>GPLGSGRPELYTVVQHVKHFNDVVEFGENQEFTDDIEYLLSGLKSTQPLNTRCLSVISLATKCAMPSFRMHLRAHGMVAMVFKTLDDSQHHQNLSLCTAALMYILSRDRLNMDLDRASLDLMIRLLELEQDASSAKLLNEKDMNKIKEKIRRLCETVHNKHLDLENITTGHLAMETLLSLTSKRAGDWFKEELRLLGGLDHIVDKVKECVDHLSRDEDEEKLVASLWGAERCLRVLESVTVHNPENQSYLIAYKDSQLIVSSAKALQHCEELIQQYNRAEDSICLADSKPLPHQNVTNHVGKAVEDCMRAIIGVLLNLTNDNEWGSTKTGEQDGLIGTALNCVLQVPKYLPQEQRFDIRVLGLGLLINLVEYSARNRHCLVNMETSCSFDSSICSGEGDDSLRIGGQVHAVQALVQLFLERERA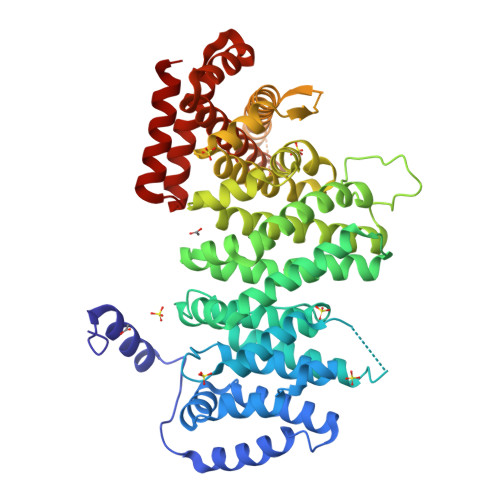AQLAESKTDELIKDAPTTQHDKSGEWQETSGEIQWVSTEKTDGTEEKHKKEEEDEELDLNKALQHAGKHMEDCIVASYTALLLGCLCQESPINVTTVREYLPEGDFSIMTEMLKKFLSFMNLTCAVGTTGQKSISRVIEYLEHC[2x]> MNSPISPIETVPVKLKPGMDGPKVKQWPLTEEKIKALVEICTEMEKEGKISKIGPENPYNTPVFA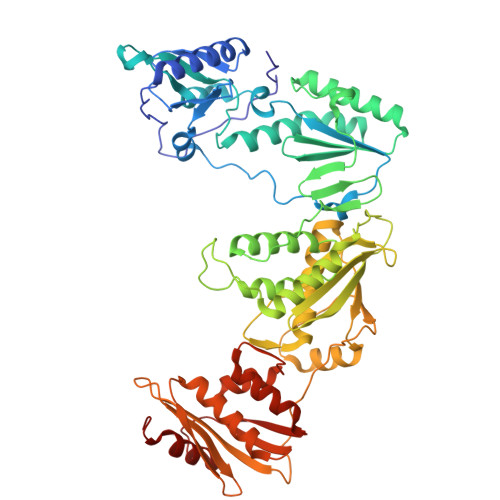IKKKDSTKWRKLVDFRELNKRTQDFWEVQLGIPHPAGLKKKKSVTVLDVGDAYFSVPLDEDFRKYTAFTIPSINNETPGIRYQYNVLPQGWKGSPAIFQSSMTKILEPFRKQNPDIVIYQYMDDLLVGSDLEIGQHRTKIEELRQHLLRWGLTTPDKKHQKEPPFLWMGYELHPDKWTVQPIVLPEKDSWTVNDIQKLVGKLNWASQIYPGIKVRQLCKLLRGTKALTEVIPLTEEAELELAENREILKEPVHGVYYDPSKDLIAEIQKQGQGQWTYQIYQEPFKNLKTGKYARMRGAHTNDVKQLTEAVQKITTESIVIWGKTPKFKLPIQKETWETWWTEYWQATWIPEWEFVNTPPLVKLWYQLEKEPIVGAETFYVDGAANRETKLGKAGYVTNRGRQKVVTLTDTTNQKTELQAIYLALQDSGLEVNIVTDSQYALGIIQAQPDQSESELVNQIIEQLIKKEKVYLAWVPAHKGIGGNEQVDKLVSAGIRKVL>[2x]AQYEDGKQYTTLEKPVAGAPQVLEFFSFFCPHCYQFEEVLHISDNVKKKLPEGVKMTKYHVNFMGGDLGKDLTQAWAVAMALGVEDKVTVPLFEGVQKTQTIRSASDIRDVFINAGIKGEEYDAAWNSFVVKSLVAQQEKAAADVQLRGVPAMFVNGKYQLNPQGMDTSNMDVFVQQYADTVKYLSEKK

The highly oxidising protein DsbA catalyses disulfide bond formation between two cysteine residues of unfolded substrates in the periplasm of Gram-negative bacteria. The structure of DsbA is comprised of a thioredoxin domain with an inserted helical domain. Like many other thiol-disulfide oxidoreductase enzymes, the active site of DsbA is comprised of the characteristic CXXC motif (Cys30–Pro31–His32–Cys33 in Escherichia coli DsbA) and a highly conserved cis-proline in an adjacent loop which has been shown to play a key role in the binding of substrates. Adjacent to the active site is a hydrophobic groove which serves as a site for both DsbB and unfolded substrates to form a complex.

Phenyl ether 25 bound to the EcDsbA groove neighbouring the active site showing a binding pose to the benzyl ether 23 and the direct anilino analogue 15. The co-structure was more comparable with the direct anilino analogue 15. The phenoxy group of 25 occupied the hydrophobic end of the binding groove with the oxygen atom of the ether linker at a distance of 4.1 Å from Gln35. The side chain of Gln35 is conformationally flexible in the crystal structure and therefore unlikely to form a hydrogen bond with 25. The carboxyl group of 25 is positioned more closely to the imidazole side chain of His32 (N–O distance = 3.7Å) compared to that of 15 (N–O distance = 4.5Å) and possibly formed a weak polar interaction. The strongest binding affinities were observed for 6-phenoxy 25 and 6-benzyl 28 with KD values of 326 ± 25 µM and 341 ± 47 µM, respectively. The similar binding affinities observed for 25 and 28 suggested that the oxygen atom of the ether linker does not contribute to the interaction, which is consistent with what we observed in the co-crystal structures. LE values showed 6-phenoxy 25 and 6-benzyl 28 were the most efficient binders.The RNA genome sizes of LSV1 and LSV2 are ~5.6 kb, encoding three major genes: the Orf1 with the unclear function, RdRP responsible for viral RNA replication, and the capsid protein (CP) for the host recognition and viral capsid assembly. CP forms the capsid shell that protects genomes and is responsible for both host specificity and receptor binding to transport the viral genome into infected host cells, or for intracellular trafficking. We determine cryo-EM structures of T = 4 and T = 3 capsids of virus-like particles (VLPs) of Lake Sinai virus (LSV) 2 and delta-N48 LSV1, belonging to tetraviruses, at resolutions of 2.3–2.6 Å in various pH environments. Analyses of these capsid structures reveal the intermolecular interactions that drive subunits assembly into homo-trimeric capsomeres and eventually into a complete viral capsid in which specific domains, such as the N-terminal domain, the helical domain, and the β-barrel domain/C-arm, could encapsidate nucleic acids.

The models of T = 4 and T = 3 LSV2 VLPs were built and refined with the homo-trimeric subunits A/B/C or D/D/D. Each icosahedral asymmetric unit (iASU) of the T = 4 particle consists of four subunits A, B, C, and D, whereas one iASU of the T = 3 particle comprises A, B, and C subunits with the C/C dimer taking up a position similar to the C/D dimer of T = 4 particles. Accordingly, the T = 4 LSV2 VLP is an icosahedral symmetrical sphere consisting of 240 copies of the 57-kDa full-length CP with 80 apparent trimeric spikes on the VLP surface, whereas the T = 3 LSV2 VLP is composed of 180 copies with 60 trimeric spikes. Besides the overall differences in VLP diameters and CP numbers, the local difference in T = 4 and T = 3 architectures is that the icosahedral 2-fold (I2) axes in T = 4 particles exist between subunits B, C, and D in two sets in the quasi six-fold (Q6) arrangement but I2 axes in T = 3 particles are present along the C/C homo-dimeric capsomeres. As a result, the T = 4 and T = 3 particle sizes of LSV2 VLP are variable, with diameters ranging from 494 to 482 Å and 450 to 438 Å, respectively, from alkaline (pH 8.5) to acidic (pH 6.5) conditions. In comparison to the expanded T = 4 and T = 3 particles at the neutral or basic pH condition, measurements of diameters of the shaped holes on the I5 and I2 axes of the unexpanded particles at pH 6.5 show that the minimum and maximum displacements were changed from ~5 to 4 Å and from ~22 to 15.5 Å, respectively. At a neutral or basic pH environment, homo-trimeric subunits A/B/C rotate along I5 axes; homo-trimeric subunits D/D/D raise around I2 axes, leading the iASU to pivot upward. In contrast, the basis of the quaternary change on the T = 4 and T = 3 particles at acidic pH is further flattened on the I2 and I3 axes, respectively, suggesting flattened hexameric capsomeres concomitantly result in a compact particle.

>[3x]MNPPTTTTTTTRTIRAPKVQLTPNSATRRRRNRRRRRPAAAIAGPLSIQPSSINRRMVSRVTRRSAVVTAAGLAWLRQYLNPMGPDTTSVTGYPDGSAVTTCIADYSNTFNVSFPPREALYCTGSSSSEKPTLVDADNYAKIDKWSNYDITLCVLALPMLRNVVMLRLYPHTPTAFALTEQTPNFPQRFPNWSVYSADGTRFNNGDEPGYLQSYVYLPNVDKHLSAARGYRLLSRGITGIFSAPALETQGFVTACQYLAEGSIQSQSIKSDAVRSVTVNSDGTVKNVESSSQTVSSMPRYVFPLDGDNCAPSSLTETYHQAYQSKATDGFYMPVLSSSRDNPFHPPQPRAIAVYGSFLARGCLDPVSEAHEADGPTHDIYRLNVADDVAPLFNTGVVWFEGISPKFSLKLKTRTVLQYIPTSGSVLANFTRHEPTYDQIALDAADRLRNLMPHAYPAAYNDWGWLGDLLDSAISMLPGVGTVYNIAKPLIKPAWNWLGNKVSDFFGNPVARDGDIFFDAK> TKVVEISPTTRLEGHSKLTLKVNDQGIVERGDWLSITPVRGIEKLAIGKTMEQVPKIASRVCGICPIAHTLASTEAMEASIGCEIPTDAKLLRIILHAANRIHSHALHNILILPDFYIPGTEKKFNLFANEQPARSVMARIVRIREIAQTIAAIAGGEAIHPSNPRIGGMYHNVSPRAKQKMADLAKECLVLVHEQMEFMLDVIRNMQNREFVEVGGKQIPLPKKLGYHNQGVMATAPMYGSSSLDDNPTWDFTRWKETRPWDWYMGEVTIDLEDPSYPIGGTTKVGTKANPQMESCTGVPTYDGQPVEVGPRARLATFKNFDEKGTFAQHIARQMEYPDCCYTI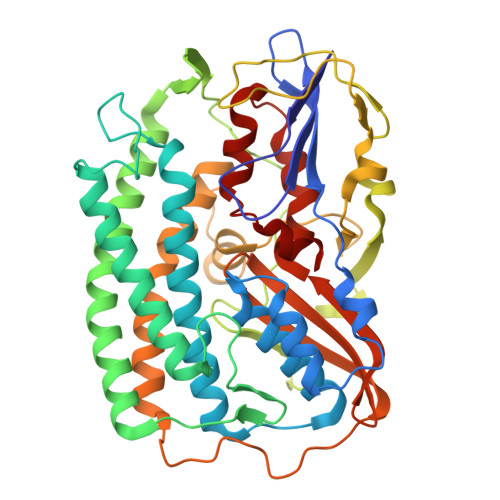LNCLDNLNTSGKVLADHIPQGDGSMGWAANEAPRGSNIHLARVKDGKVRWYDMLVPTTWNFPTCSRALTGAPWQIAEMVVRAYDPCVSCATH>[2x]MGHELEVDIEPKKTPENPEYDNEIEATNSVIIAGYGRFG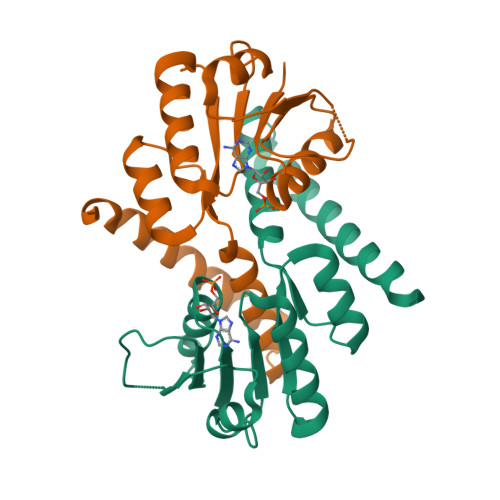QVVGRLLSAQGYHLSILDHSPSQIDMLRRFGNKVFYGDAARKDLLEAAGAKDAQLLVIAIDAPDKALEIVELAHKHYPQLKIVARAIDRRHAYQYLRLGVTSFKRETFDSAVNLGIEALTLLGNSSTVAERAGDLFSQHDNASLHELAALWGDDHTYGVAVRQRMEDLKQVLAKDKAAQERLNTCKGGDCLEHHHHHH>MAPRKFFVGGNWKMNGDKKSLGELIHTLNGAKLSADTEVVCGAPSIYLDFARQKLDAKIGVAAQNCYKVPKGAFTGEISPAMIKDIGAAWVILGHSERRHVFGESDELIGQKVAHALAEGLGVIACIGEKLDEREAGITEKVVFEQTKAIADNVKDWSKVVLAYEPVWA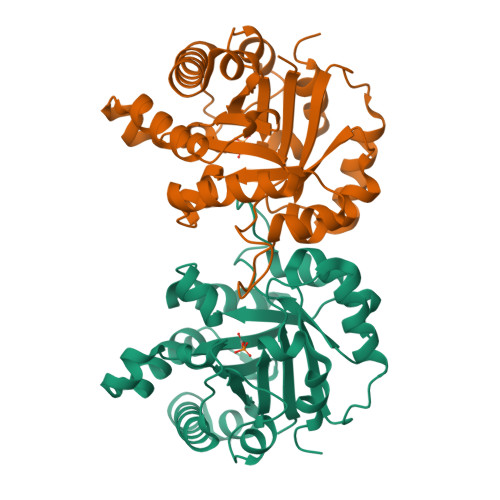IGTGNSSTPQQAQEVHEKLRGWLKSHVSDAVAQSTRIIYGGSVTGGNCKELASQHDVDGFLVGGASLKPEFVDIINAKH[2x]>[2x]MEDVEIKPRGYQLRLVDHLTKSNGIVYLPTGSGKTFVAILVLKRFSQDFDKPIESGGKRALFMCNTVELARQQAMAVRRCTNFKVGFYVGEQGVDDWTRGMWSDEIKKNQVLVGTAQVFLDMVTQTYVALSSLSVVIIDECHHGTGHHPFREFMRLFTIANQTKLPRVVGLTGVLIKGNEITNVATKLKELEITYRGNIITVSDTKEMENVMLYATKPTEVMVSFPHQEQVLTVTRLISAEIEKFYVSLDLMNIGVQPIRRSKSLQCLRDPSKKSFVKQLFNDFLYQMKEYGIYAASIAIISLIVEFDIKRRQAETLSVKLMHRTALTLCEKIRHLLVQKLQDMTYDDDDDNVNTEEVIMNFSTPKVQRFLMSLKVSFADKDPKDICCLVFVERRYTCKCIYGLLLNYIQSTPELRNVLTPQFMVGRNNISPDFESVLERKWQKSAIQQFRDGNANLMICSSVLEEGIDVQACNHVFILDPVKTFNMYVQSKGRARTTEAKFVLFTADKEREKTIQQIYQYRKAHNDIAEYLKDRVLEKTEPELYEIKGHFQDDIDPFTNENGAVLLPNNALAILHRYCQTIPTDAFGFVIPWFHVLQEDERDRIFGVSAKGKHVISINMPVNCMLRDTIYSDPMDNVKTAKISAAFKACKVLYSLGELNERFVPKTLKERVASIADVHFEHWNKYGDSVTATVNKADKSKDRTYKTECPLEFYDALPRVGEICYAYEIFLEPQFESCEYTEHMYLNLQTPRNYAILLRNKLPRLAEMPLFSNQGKLHVRVANAPLEVIIQNSEQLELLHQFHGMVFRDILKIWHPFFVLDRRSKENSYLVVPLILGAGEQKCFDWELMTNFRRLPQSHGSNVQQREQQPAPRPEDFEGKIVTQWYANYDKPMLVTKVHRELTPLSYMEKNQQDKTYYEFTMSKYGNRIGDVVHKDKFMIEVRDLTEQLTFYVHNRGKFNAKSKAKMKVILIPELCFNFNFPGDLWLKLIFLPSILNRMYFLLHAEALRKRFNTYLNLHLLPFNGTDYMPRPLEIDYSLKRNVDPLGNVIPTEDIEEPKSLLEPMPTKSIEASVANLEITEFENPWQKYMEPVDLSRNLLSTYPVELDYYYHFSVGNVCEMNEMDFEDKEYWAKNQFHMPTGNIYGNRTPAKTNANVPALMPSKPTVRGKVKPLLILQKTVSKEHITPAEQGEFLAAITASSAADVFDMERLEILGNSFLKLSATLYLASKYSDWNEGTLTEVKSKLVSNRNLLFCLIDADIPKTLNTIQFTPRYTWLPPGISLPHNVLALWRENPEFAKIIGPHNLRDLALGDEESLVKGNCSDINYNRFVEGCRANGQSFYAGADFSSEVNFCVGLVTIPNKVIADTLEALLGVIVKNYGLQHAFKMLEYFKICRADIDKPLTQLLNLELGGKKMRANVNTTEIDGFLINHYYLEKNLGYTFKDRRYLLQALTHPSYPTNRITGSYQELEFIGNAILDFLISAYIFENNTKMNPGALTDLRSALVNNTTLACICVRHRLHFFILAENAKLSEIISKFVNFQESQGHRVTNYVRILLEEADVQPTPLDLDDELDMTELPHANKCISQEAEKGVPPKGEFNMSTNVDVPKALGDVLEALIAAVYLDCRDLQRTWEVIFNLFEPELQEFTRKVPINHIRQLVEHKHAKPVFSSPIVEGETVMVSCQFTCMEKTIKVYGFGSNKDQAKLSAAKHALQQLSKCDA;>[2x]MDQENFHGSSLPQQLQNLHIQPQQASPNPVQTGFAPRRHYNNLVGLGNGNAVSGSPVKGAPLGQRHVKLKKEKISAQVAQLSQPGQLQLSDVGDPALAGGSGLQGGVGLMGVILPSDEALKFVSETDANGLAMKTPVSILQELLSRRGITPGYELVQIEGAIHEPTFRFRVSFKDKDTPFTAMGAGRSKKEAKHAAARALIDKLIGAQLPESPSSSAGPSVTGLTVAGSGGDGNANATGGGDASDKTVGNPIGWLQEMCMQRRWPPPSYETETEVGLPHERLFTIACSILNYREMGKGKSKKIAKRLAAHRMWMRLQETPIDSGKISDSICGELEGEVSIIQDIDRYEQVSKDFEFIKI

In Drosophila, an RNase III enzyme Dicer-2 (Dcr-2), aided by its cofactor Loquacious-PD (Loqs-PD), has an important role in generating 21 bp siRNA duplexes from long double-stranded RNAs (dsRNAs). ATP hydrolysis by the helicase domain of Dcr-2 is critical to the successful processing of a long dsRNA into consecutive siRNA duplexes. Here six cryo-electron microscopy (cryo-EM) structures of Drosophila Dcr-2–Loqs-PD in apo and in complex with dsRNA substrate in the absence or in the presence of ATP were captured, illuminating the continuous conformational changes of Dcr-2–Loqs-PD after binding to dsRNA and translocating until forming the active dicing state and cleaving the dsRNA substrate into an siRNA duplex in the post-dicing state. Loqs-PD is a cofactor protein that comprises two dsRBDs that are responsible for recruiting siRNA precursor substrates for Dcr-2.

To capture the different steps during the translocation of Dcr-2–Loqs-PD along the dsRNA, we used cryo-EM to analyse the sample of Dcr-2DDNN–Loqs-PD in complex with the dsRNA substrate under conditions with ATP and Mg2+. Through single-particle classification, we captured two representative cryo-EM structures of Dcr-2–Loqs-PD in complex with the dsRNA substrate in translocation states. We captured another structure in the mid-translocation state, in which about 17 bp of a dsRNA duplex threads through the helicase domain further towards the catalytic centre of Dcr-2. When superimposed onto structures of the initial binding and early translocation states, the cap–core modules sway back about 2 Å towards the dsRNA. Importantly, in the mid-translocation state, the C-terminal dsRBD of Dcr-2 appears in the map and interacts with the dsRNA substrate, resulting in further bending of the axis of the dsRNA about 25°, and the trajectory of the dsRNA is directly towards the PAZ domain. During the translocation, the interactions between the DUF283 domain and RIIIDa/b domains, including relatively flexible interactions between the DUF283 and RIIIDb/RIIIDbi domains, and relatively rigid interactions between the DUF283 domain and RIIIDa through the DP-linker domain, remain almost the same as in the initial binding state. This suggests that the overall domain configuration of Dcr-2 is relatively rigid during the translocation process until the dsRNA terminus reaches the Platform–PAZ domains. A comparison of the cryo-EM structures of the early- and mid-translocation states also demonstrates a very similar structure in their helicase domains, of which the ATP-hydrolytic pockets have an EM density for either ATP or ADP-Mg2+. Moreover, DUF283 interacts with RIIIDb and RIIIDa, blocking the access of dsRNA to the catalytic centre of RIIIDa/b and preventing non-specific cleavage of dsRNA during the translocation.> GAMGQTSTRWTPTTEQIKILKELYYNNAIRSPTADQIQKITARLRQFGKIEGKNVFYWFQNHKARERQKKRFNGGS

The HD transcription factor WUS plays key roles for plant development with at least four distinct and essential subfunctions: Firstly, regulation of stem cell identity in the shoot apical meristem (SAM), where it is required for non cell-autonomous induction and maintenance of stem cell fate via stimulation of cytokinin and suppression of auxin signaling. Consistent with a broad functional portfolio, WUS has been shown to bind to a diverse set of DNA motifs in the regulatory regions of downstream genes involved in SAM development and signaling processes. Here, we have combined molecular, biochemical, and structural approaches to address how the WUS-HD recognizes specific DNA target sites. We find that the DNA-binding preferences of WUS-HD depend on appropriately arranged sequence motifs in a direct tandem repeat and that homodimerization is one of the key determinants to achieve high sequence specificity.

As an entry point to elucidate the mechanisms by which the WUS-HD carries out its functions, we recombinantly produced and purified a fragment containing residues 34–103 of WUS and determined its crystal structure to a resolution of 1.4 Å. The overall WUS-HD fold reflected that of a canonical HD structure, consisting of a three-helix bundle with an N-terminal arm. Interestingly, superposition with the structure of Engrailed (En) (PDB code 3HDD23) and comparative sequence analyses identified unique structural features in WUS-HD. First, the loop regions connecting the three α-helices are expanded. Loop region I is slightly longer compared to other HDs and is characterized by a distortion at the end of helix α1. This so called π-helix or π-bulge is typically characterized by a single amino acid insertion into an existing α-helix (Y54 in WUS) and usually correlates with a particular functional role. Loop region II has an even longer insertion, which also extends helix α2 by an additional turn compared to En. Secondly, the N-terminal arm is anchored by docking of a tryptophan residue (W39) into a groove formed by helices α2 and α3, while a F, Y, or I residue typically performs this function in canonical HDs. Furthermore, this docking residue is shifted by one residue relative to the conserved DNA-contacting arginine (R38) in contrast to three residues in canonical HDs. Electrostatic surface calculations showed a large positively charged surface formed by the C-terminal recognition helix (α3) and the N-terminal arm, which represent the most conserved part of the HD.> GPGSVDTERPVVDFPGEINVYRGESFEFIATATDNSNAFDINKTYVRWYNGTDSGRGTEWIEKTVTQEGNLLKVKVHGKVPVDTDIGHYTRYVMVTDAAGNQNVSNEEFSAALTNKDRILNGQFRIVIRYRPNLPENTVLVNNPSQLSETEKNQVREAIKQSNPNLRPIDVAGKNLDTAISVSNNGTTTITFRDNRKATIQGKDLVDTRAGS

Many streptococci adhere to protein-attached carbohydrates expressed on cell surfaces using Siglec-like binding regions (SLBRs). Siglec-like binding regions (SLBRs) are among the streptococcal adhesive modules that bind sialoglycans. SLBRs contain two adjacent modules: a Siglec domain, which shares some features with mammalian Siglecs, and a Unique domain13 with no close homologs outside of the family. The conserved sialic acid-recognition motif governs general specificity while sequence diversity in surrounding loop regions allows the SLBR to select between related sialoglycans.

We identified that a previously-uncharacterized SLBR from Streptococcus sanguinis strain SK150 (termed SLBRSK150) displays 62% identity to SLBRGspB but exhibits a distinct binding profile. In short, there was modest binding to each of the three trisaccharides, i.e., sTa, 3’sLn, and sLeC, but little detectable binding to any of the tetrasaccharides (i.e., 6S-sLeX, sialyl Lewis X (sLeX; Neu5Acα2-3Galβ1-4(Fucα1-3)GlcNAcβ; Fig. 1d), and sialyl LewisA (sLeA; Neu5Acα2-3Galβ1-3(Fucα1-4)GlcNAcβ; Fig. 1e)). The high sequence similarity and distinct binding properties of SLBRGspB and SLBRSK150 make these good comparators for understanding selectivity. To reveal how similar SLBRs could include or exclude different sialoglycans, we determined crystal structures of these five SLBRs at resolutions between 1.0 Å and 1.7 Å. We next turned to SLBRGspB and SLBRSK150, which both bind sTa preferentially.>[2x]DAAQPALLQYHYDCGDFGMQLLAYPTRGRTVHFKVLDEFGTRFEVANCSICMHWLNTGEDGGLIFSAGYEGCHVLVKDGRYVLRVQLEEMLLSGVVAASYEVQMTCPRPAGYEILRDEKVHH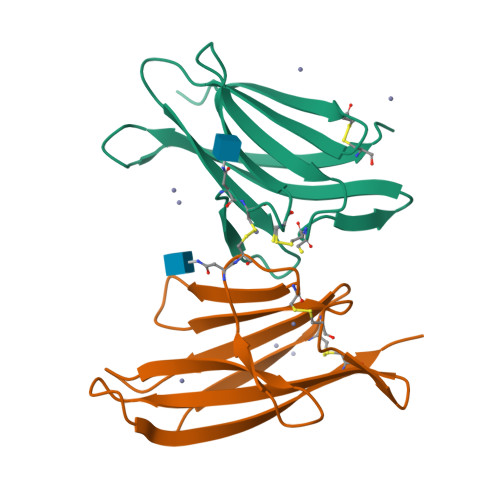HHHHHHQRPDRGNS> LGGVDREAMARCIEECLRCAQACTACADACLSEPAVADLTKCIRTDMDCA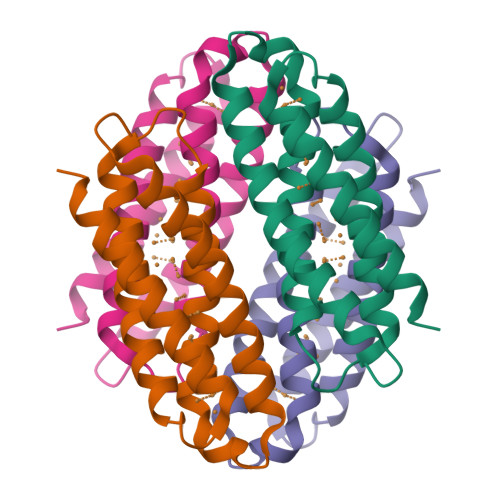DVCTATAAVLSRHTGYDANVTRAVLQACATVCAACGDECARHAGMHEHCRVCAEACRSCEQACQELLAGLG The structures of two major GSTs, Na-GST-1 and Na-GST-2 from Necator americanus, have been determined using recombinant protein expressed in and secreted by Pichia pastoris. GSTs are homodimers that catalyze the nucleophilic addition of reduced glutathione to various diverse electrophilic substrates consequently facilitating their inactivation, and extrusion. GSTs are a major detoxification system for helminths, which have limited detoxification enzymes and apparently lack the cytochrome P-450 dependent reactions. The fundamental/active units of both structures are homodimers with the classical GST topology of Nu class nematode specific GSTs.

The orthorhombic Na-GST-1 contains a tetramer per asymmetric unit which corresponds to a Matthews' coefficient of 2.3 Å/Da and solvent content of 46%. The primary and tertiary structures of Na-GST-1 are more like that of HpolGST than Na-GST-2. All the main chain atoms for all 206 amino acids for all monomers were ordered in the Na-GST-1 structures however some monomers have disordered side chain residues, most prominently in the region from amino acids 105 through 132, interestingly these residues are include some of those that break the higher order symmetry of the Na-GST-2 structure. No such density was observed in the electron density maps for Na-GST-1, instead scattered density were visible in the substrate binding cavity. Interestingly, the G-site of Na-GST-1 cannot fit glutathione as it is abrogated by Gln 50 which points directly in the binding cavity blocking glutathione binding. A rotation of Gln around the Cβ will allow sufficient room for gluthatione to bind. It is plausible that a pH change may facilitate this rotation. Na-GST-1 was crystallized at an acidic pH 4.6 whereas Na-GST-2 was crystallized at a more basic pH of 7.5. Evidently, Na-GST-1 is capable of binding glutathione and like Na-GST-2 is catalytically active at pH 6.8 as measured by glutathione conjugation with 1-chloro-2, 4-dinitrobenzene (CDNB). Furthermore, the cavity is more open in the absence of glutathione (in the case of Na-GST-1) than with glutathione bound (in the case of Na-GST-2), suggesting a conformational variation upon glutathione binding.

>[4x]MVHYKLTYFAIRGAGECARQIFALADQEFEDVRLDKEQFAKVKPDLPFGQVPVLEVDGKQLAQSLAICRYLARQFGFAGKSTFDEAVVDSLADQYSDYRVEIKSFFYTVIGMREGDVEQLKKEVLLPARDKFFGFITKFLKKSPSGFLVGDSLTWVDLLVSEHNATMLTFVPEFLEGYPEVKEHMEKIRAIPKLKKWIETRPETLF>MRGSHHHHHHGMASMRILLSNDDGVHAPGIQTLAKALREFADVQVVAPDRNRSGASNSLTLESSLRTFTFDNGDIAVQMGTPTDCVYLGVNALMRPRPDIVVSGINAGPNLGDDVIYSGTVAAAMAGRHLGFPALAVSLNGYQHYDTAAAVTCALLRGLSREPLRTGRILNVNVPDLPLAQVKGIRVTRCGSRHPADKVIPQEDPRGNTLYWIGPPGDKYDAGPD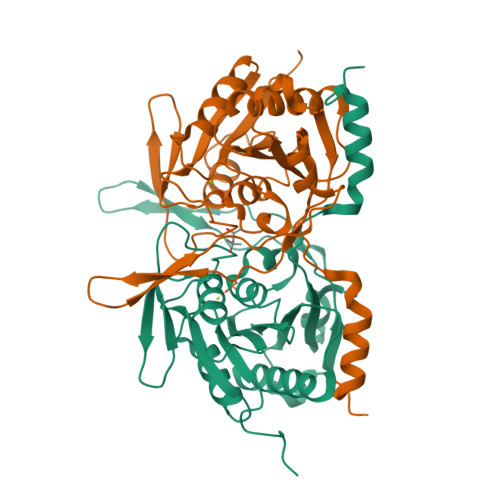TDFAAVDEGYVSVTPLHVDLTAASAHDVVSDWLDSVGVGTQW[4x]(2R)-N-hydroxy-2-methyl-2-(methylsulfonyl)-4-{4'-[3-(morpholin-4-yl)propoxy]biphenyl-4-yl}butanamide | C25 H34 N2 O6 S | 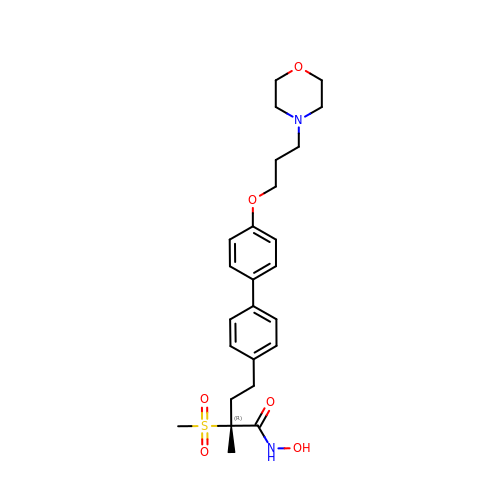GGIDQMXKOSYOHO-RUZDIDTESA-N> CKRPRPEGMQTLESFFKPLT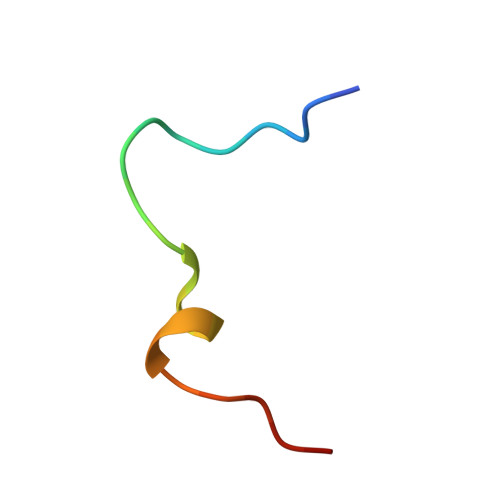H> MAQIVDVYGNPIRTQQLREPQTSRLAGLAKEFAQHPAKGLTPAKLARILVEAEQGNLQAQAELFMDMEERDAHLFAEMSKRKRAILGLDWAVEPPRNASAAEKADADYLHELLLDLEGLEDLLLDALDGIGHGYSCIELEWALQGREWMPLAFHHRPQSWFQLNPEDQNELRLRDNSPAGEALQPFGWIIHRPRARSGYVARSGLFRVLAWPYLFRHYATSDLAEMLEIYGLPIRLGKYPPGTADEEKATLLRAVTGLGHAAAGIIPETMAIDFQQAAQGSSDPFLAMMRQSEDAISKAVLGGTLTSTTSQSGGGAFALGQVHNEVRHDLLASDARQLAATLSRDLLWPLLVLNRPGSPDVRRAPRLVFDLREQADITSMAQSIPALVNVGLEIPSAWVYDKLGIPQPAKNEPVLRSAAQPAILSRQHGQRVAALATIVGPRYGDQQALDKALASLPAKDMQDQVNDLLAPLLEAVNRGDSETELLGALAEAFPDMDDSALTDALHRLLFAADTWGRLHGNLDRID;> MSYCTLADLIEQYSEQKIREVSDRVNKPATTIDTVIVD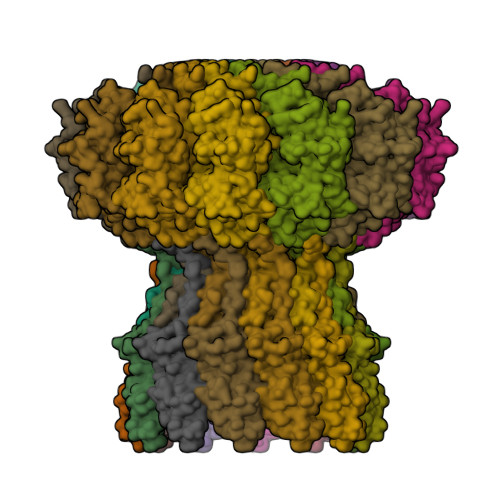RAIADADSEIDLHLHGRYQLPLASVPTALKRIACGLAYANLHIVLKEENPVYKTAEHLRKLLSGIANGKLSLALDADGKPAPVANTVQISEGRNDWGADW>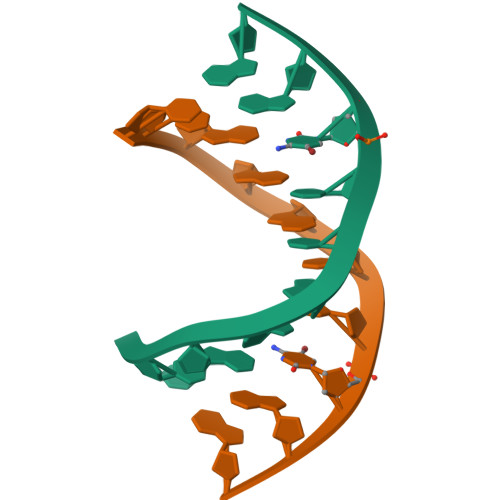[2x]CCGGGCCCGG Aurora A kinase (AURKA) is a member of a family of Ser/Thr kinases whose orthologues control progression through mitotic cell division. The localisation of AURKA to microtubules in the mitotic spindle is mediated through its interaction with a protein partner, TPX227. Besides localisation, the AURKA-TPX2 interaction modulates the catalytic activity of AURKA3738. Here, we report the identification of AurkinA, a drug-like inhibitor of AURKA, which binds to a pocket occupied by Y8 and Y10 of TPX2 in the AURKA-TPX2 complex (the Y-pocket).

To provide structural insight into how AurkinA binding might hinder formation of the AURKA-TPX2 complex, we determined the crystal structures of the AURKA catalytic domain in isolation or when liganded to AurkinA. We noted that whilst the structure for AA30, like that for AurkinA could be determined in complex with AURKA bound either to Mg2+-ATP or JNJ-7706621 in the active site, the AA29 compound could only be soaked into AURKA complexed with JNJ-7706621. Interestingly, depending on the concentration of reducing agent in buffer, the AURKA kinase domain crystallised either in space group P6122 or in P41212. In contrast, the binding of AurkinA, and indeed any of our compounds increased the overall B-factors of the crystal structures. Importantly, in all structures where a small molecule is bound in the Y-pocket, the electron density for the AURKA activation loop remained largely undefined. More detailed analysis of the liganded crystal structures revealed that binding of AurkinA and its analogues caused significant local alterations to AURKA structure, as well as changes at sites distant from the Y-pocket. Based on our structural data, we hypothesised that the allosteric, Y-pocket-binding inhibitors would not affect the Km for ATP, as no significant changes in residues involved in ATP binding directly were observed upon AurkinA binding and ATP was always present in the active site. The F165-F144 backbone hydrogen bond was significantly shortened (3.2 Å to 2.8 Å) and the K143-Q168 hydrogen bond present in the ‘active’ apo structure was broken in the presence of the Y-pocket binders, potentially impairing the ADP removal from the ATP-site.

> MGRQWALEDFEIGRPLGKGKFGNVYLAREKQSKFILALKVLFKAQLEKAGVEHQLRREVEIQSHLRHPNILRLYGYFHDATRVYLILEYAPLGTVYRELQKLSKFDEQRTATYITELANALSYCHSKRVIHRDIKPENLLLGSAGELKIADFGWSVHAPSSRRATLCGTLDYLPPEMIEGRMHDEKVDLWSLGVLCYEFLVGKPPFEANTYQETYKRISRVEFTFPDFVTEGARDLISRLLKHNPSQRPMLREVLEHPWITANSSKPHHHHHH> MEHHHHHHMPVFHTRT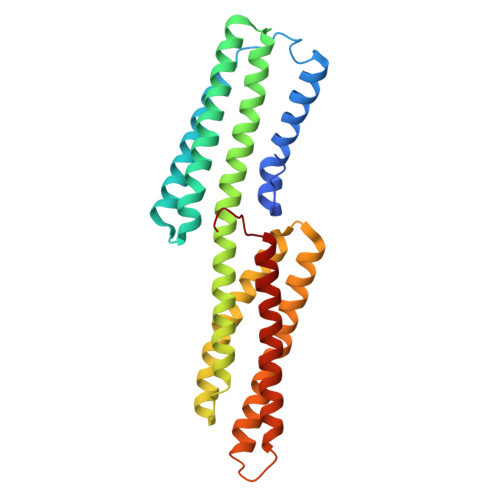IESILEPVAQQISHLVIMHEEGEVDGKAIPDLTAPVAAVQAAVSNLVRVGKETVQTTEDQILKRDMPPAFIKVENACTKLVQAAQMLQSDPYSVPARDYLIDGSRGILSGTSDLLLTFDEAEVRKIIRVCKGILEYLTVAEVVETMEDLVTYTKNLGPGMTKMAKMIDERQQELTHQEHRVMLVNSMNTVKELLPVLISAMKIFVTTKNSKNQGIEEALKNRNFTVEKMSAEINEIIRVLQLTSWDEDAW>MKPVKPPRINGRVPVLSAQEAVNYIPDEATLCVLGAGGGILEATTLITALADKYKQTQTPRNLSIISPTGLGDRADRGISPLAQEGLVKWALCGHWGQSPRISDLAEQNKIIAYNYPQGVLTQTLRAAAAHQPGIISDIGIGTFVDPRQQGGKLNEVTKEDLIKLVEFDNKEYLYYKAIAPDIAFIRATTCDSEGYATFEDEVMYLDALVIAQAVHNNGGIVMMQVQKMVKKATLHPKSVRIPGYLVDIVVVDPDQSQLYGGAPVNRFISGDFTLDDSTKLSLPLNQRKLVARRALFEMRKGAVGNVGVGIADGIGLVAREEGCADDFILTVETGPIGGITSQGIAFGANVNTRAILDMTSQFDFYHGGGLDVCYLSFAEVDQHGNVGVHKFNGKIMGTGGFIDISATSKKIIFCGTLTAGSLKTEIADGKLNIVQEGRVKKFIRELPEITFSGKIALERGLDVRYITERAVFTLKEDGLHLIEIAPGVDLQKDILDKMDFTPVISPELKLMDERLFIDAAMGF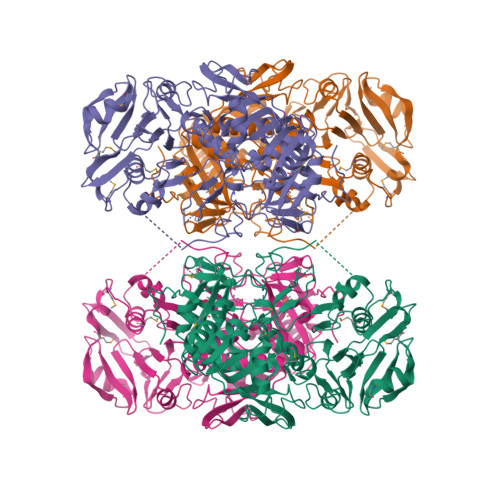VLPEAAH[4x]>[24x]MRKFLKVTLASALIGCGVIGTVSSLMVKEAKAVEIITHWVPHEVYGMPGEPDNSGKVFFSGLKAKYMGYPKDAQRSPYPGKYSKFWKTLPAYRYYIPDYMYNRDEVRPSNPIKGTFKLEQCVACHSVMTPGIVRDYNKSAHSKAEPAPTGCDTCHGNNHQKLTMPSSKACGTAECHETQYNEQGQGGIGSHASCSSFAQVECAWSIERPPGDTAGCTFCHTSPEERCSTCHQRHQFDPAVARRS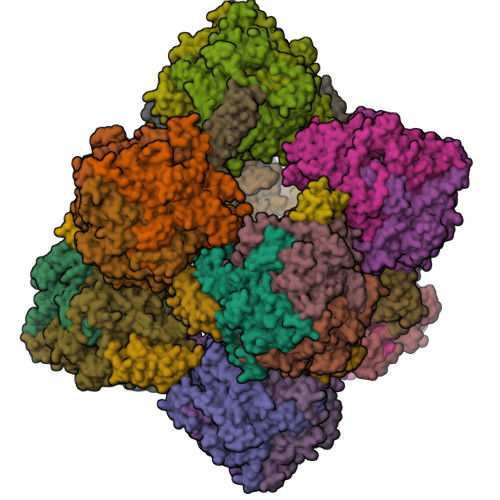EQCKTCHWGKDHRDWEAYDIGLHGTVYQVNKWDTEQFDFSKKLSDADYVGPTCQYCHMRGGHHNVQRASIVYTSMGMSMADRGAPLWKEKRDRWVSICDDCHSPRFARENLQAMDESVKDASLKYRETFKVAEDLLIDGVLDPMPKDLCPDWSGQHIWSLKIGAYHDGEAYGGTTGESGEFRMSNCTDVERLCFESVGYFQTYIYKGMAHGSWNDATYSDGSFGMDRWLVNVKQNASRARRLAALEKKVGISWQPEQFWKTGEWLDQLTGPYIVKNHPGKTIFDLCPDPGWLDTHHAPAEEVEYIERKLKELGITAGSHSAHHHESGHDPAARSMKEH;>[12x]MLKKVLVGMFGAALIAGIGMTTAQAYDVKPAKLWVTAIAIGTPIVGAEIKVGDEECTTGNNGTCVFELRPGTYAISVHEHGGQSAHKEVSLEEGNILFVSLDLGAKARHPSGSH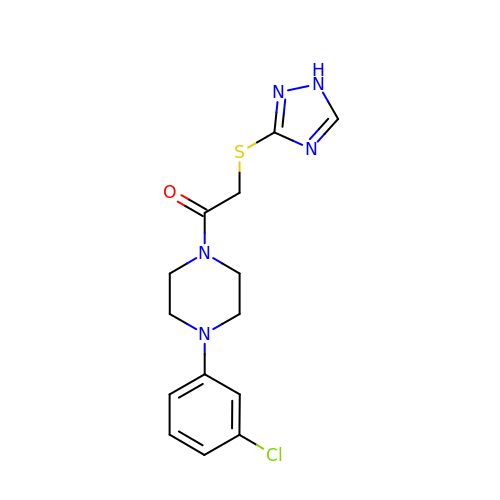2-((4H-1,2,4-triazol-3-yl)thio)-1-(4-(3-chlorophenyl)piperazin-1-yl)ethan-1-one | C14 H16 Cl N5 O S | RMTODJAENUIFJI-UHFFFAOYSA-N>[2x]HHHHHHDESSDPGPQHRVQGPGPEPTLGPLTRLEGIKVGHERKVQLVTDRDHFIRTLSLKPLLFEIPGFLTDEECRLIIHLAQMKGLQRSQILPTEEYEEAMSTMQVSQLDLFRLLDQNRDGHLQLREVLAQTRLGNGWWMTPESIQEMYAAIKADPDGDGVLSLQEFSNMDLRDFHKYMRSHKAESSELVRNSHHTWLYQGEGAHHIMRAIRQRVLRLTRLSPEIVELSEPLQVVRYGEGGHYHAHVDSGPVYPETICSHTKLVANESVPFETSCRYMTVLFYLNNVTGGGETVFPVADNRTYDEMSLIQDDVDLRDTRRHCDKGNLRVKPQQGTAVFWYNYLPDGQGWVGDVDDYSLHGGCLVTRGTKWIANNWINVDPSRARQALFQQEMARLAREGGTDSQPEWALDRAYRDARVEL

In addition to collagen P4Hs and hypoxia-inducible factor P4Hs, a third P4H—the poorly characterized endoplasmic reticulum–localized transmembrane prolyl 4-hydroxylase (P4H-TM)—is found in animals. All known P4Hs belong to the same enzyme superfamily of iron and 2-oxoglutarate–dependent dioxygenases (2OGDDs). P4H-TM is a functionally enigmatic enzyme that is localized at the ER membrane. It is composed of an N-terminal cytoplasmic tail, a membrane-anchoring transmembrane helix, and a unique combination of a Ca2+-binding EF domain and a catalytic domain that is located within the ER lumen. The 2OGDD protein family includes single-domain and large multidomain proteins that are highly variable in their substrate specificity, but P4H-TM is the only enzyme in this family that has EF-hand motifs.

The structure of the soluble part of human P4H-TM was solved with X-ray crystallography in the presence of Fe2+, N-oxalylglycine (NOG), and Ca2+. The crystallized construct consists of residues 88 to 502 of P4H-TM and an N-terminal His-tag, whereas it lacks the short cytoplasmic region and the transmembrane helix. The crystal structure shows that the P4H-TM fold is composed of two well-defined domains: the catalytic domain with the DSBH fold and the EF domain. There are two P4H-TM molecules in the asymmetric unit. The two P4H-TM molecules of the asymmetric unit occupy very similar conformations (RMSD 0.42 Å for all Cα-atoms), and only chain A is discussed unless otherwise stated. The P4H-TM structure contains an EF domain with two EF hands between residues 190 and 251. Calcium is coordinated in a pentagonal bipyramid conformation by seven oxygen ligands from residues listed in Table 1. The active site iron is coordinated by His328, Asp330, His441, and the oxygen atoms from C-1 carboxylate and C-2 carbonyl of NOG. NOG is coordinated at the C-5 carboxyl group by Tyr319, Thr375, and Lys451 and at the C-1 carboxyl by Asn455. In the structure, Asn368 and Asn382 were found to be glycosylated, whereas Asn348 is located in a part of the βII-βIII loop where the electron density for the side chain was not well defined. In this P4H-TM structure, the α1-α2 loop is partially disordered and positioned like a lid in an open conformation.(14S)-14-methylhexadecanoic 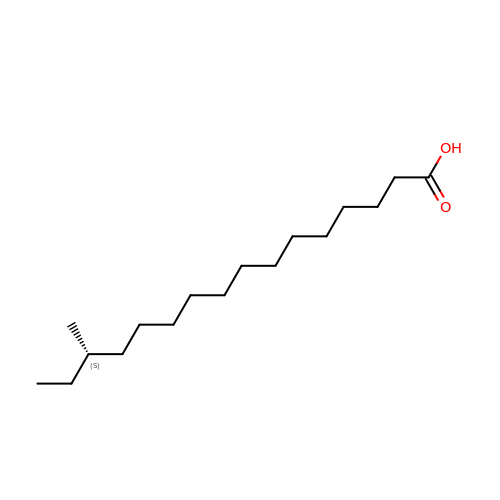acid | C17 H34 O2 | FXUKWLSZZHVEJD-INIZCTEOSA-N Here, we characterize the O-methyltransferases BelI and CysG, which catalyze the initial step of β-lactone formation. Employing techniques such as crystallography, computational analysis, mutagenesis, and activity assays, we identified a His-His-Asp (HHD) motif in the active sites of the two enzymes, which is crucial for binding a catalytically active calcium ion. As expected, BelI as well as CysGΔN16 adopt the class I methyltransferase Rossmann fold, characterized by a core domain of a seven-stranded β-sheet flanked by α-helices. The HHD-motif enables regiospecific C1-carboxy group methylation of their respective malic substrates.

Conservative asparagine replacements in the HHD motif resulted in CysG variants that remained active. CysGfl-D191N showed a 56% decrease in substrate turnover, while CysGfl-H122N and CysGfl-H123N were fully active compared to wt but were inactivated with EDTA.

>[2x]GSTYDALRRQLIPSFDLLYGSAVSVVAMSVPATARILDLGAGTGLLGAALRERLPDAELLLQDRSQAMLEQARQRFADDDQVAIRVADHLDELPAGPFDAVVSALSINHLEHQDKQDLFTRIRKILRPGGIFVNVEQVLAPTSELEKMYDRQHEAHVLASDTPAEEWAAGRERMKHDIPIDVETQIQWLRDAGFTTADCLAKDWRFATYAGWNGS> GPYTFVQQHLMIGTDPRTILKDLLPETIPPPELDDMTLWQIVINILSEPPKRKKRKDINTIEDAVKLLQECKKIIVLTGAGVSVSCGIPDFRSRDGIYARLAVDFPDLPDPQAMFDIEYFRKDPRPFFKFAKEIYPGQFQPSLCHKFIALSDKEGKLLRNYTQNIDTLEQVAGIQRIIQCHGSFATASCLICKYKVDCEAVRGDIFNQVVPRCPRCPADEPLAIMKPEI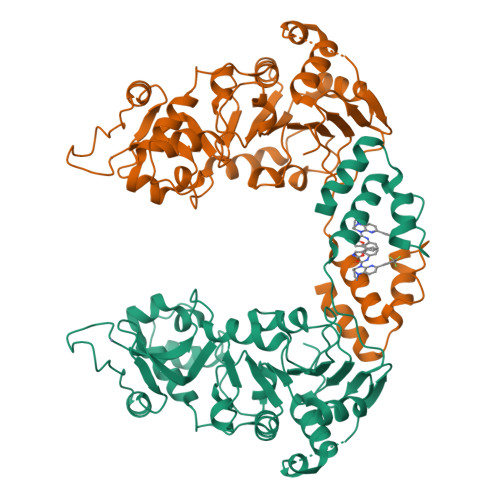VFFGENLPEQFHRAMKYDKDEVDLLIVIGSSLKVRPVALIPSSIPHEVPQILINREPLPHLHFDVELLGDCDVIINELCHRLGGEYAKLCCNPVGGGSGGGSQYLFLPPNRYIFHGAEVYSDSEDDV 N-cyclopentyladenosine 5'-(dihydrogen phosphate) | C15 H22 N5 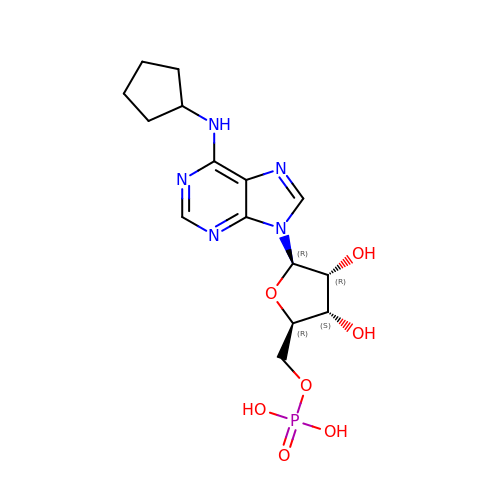O7 P | ZLXWBMMFOMQXRH-SDBHATRESA-N>[2x]HMGRSQNSEFETASDEPIAVIGLSCRLPKASG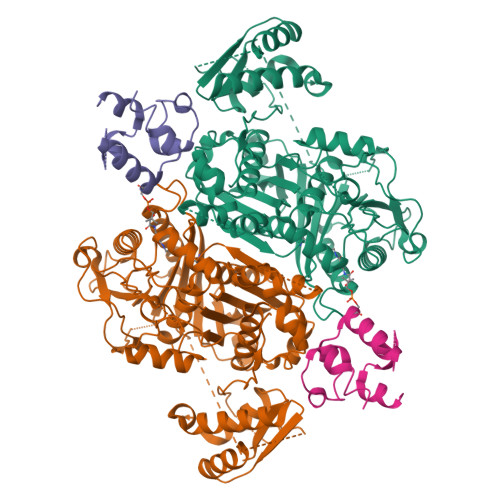PQELWQLLDDGASAVTRVPADRETPPSTEEESADGEAAGARWGGFLDRVDTFDAGFFGISPREAAAMDPQQRLVLELSWEALEGAGLVPATLRDTGLGVFVGAARDDYATLYRRREGRAVDHHAMTGLHRSLIANRISYALGAHGPSMVVDTGCSSSLVAVHLACESLRRGESDIALAGGVNLNIAAESARETAAFGGLSPDGQCFTFDARANGFVRGEGGGLVVLKTLRRALADGDLVHGVILASAVNNDGPSDTLTTPSRRAQESLLTRVYRRAGVTPTEVGYVELHGTGTKVGDPIEAAALGAVLGTGRDTPLPVGSIKTNIGHLEGAAGIAGLIKALLQLRRRRLVPSLNFSTPNPDIPLDALNLRVQQESAPWATPSGGGRTLVAGVSSFGMGGTNCHVVVSAAPVPEDGETTSEAGATGPDSGPALLPWVVSARSPQALRDQAGRLAAWADSPAGREASPVDIGWSLATSRTHFEYRAVVSGSDRDELVASLRALASGSPVTAAGAVDGRAEPVALLSAVGELFADGYPVDWTAYFAGWPAARVELPTYAFQRSRHWLENVPELAVS;>[2x]HMPREPVTPDSDHPDPVETVRQLTAHVLGLTAAADVEMTRSFKDLGFDSLMSVELRDRLCAATGLSLATTLLYDHPSPAETAEFVRARLTGDEA>[4x]MSQHNEKNPHQHQSPLHDSSEAKPGMDSLAPEDGSHRPAAEPTPPGAQPTAPGSLKAPDTRNEKLNSLEDVRKGSENYALTTNQGVRIADDQNSLRAGSRGPTLLEDFILREKIAHFDHERIPERIVHARGSAAHGYFQPYKSLSDITKADFLSDPNKITPVFVRFSTVQGGAGSADTVRDIRGFATKFYTEEGIFDLVGNNTPIFFIQDAHKFPDFVHAVKPEPHWAIPQGQSAHDTFWDYVSLQP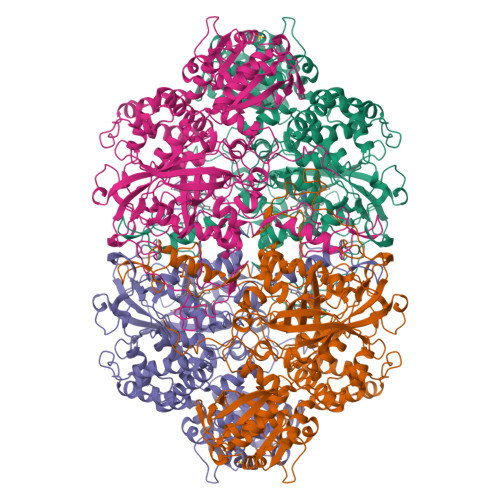ETLHNVMWAMSDRGIPRSYRTMEGFGIHTFRLINAEGKATFVRFHWKPLAGKASLVWDEAQKLTGRDPDFHRRELWEAIEAGDFPEYELGFQLIPEEDEFKFDFDLLDPTKLIPEELVPVQRVGKMVLNRNPDNFFAENEQAAFHPGHIVPGLDFTNDPLLQGRLYSYTDTQISRLGGPNFHEIPINRPTCPYHNFQRDGMHRMGIDTNPANYEPNSINDNWPRETPPGPKRGGFESYQERVEGNKVRERSPSFGEYYSHPRLFWLSQTPFEQRHIVDGFSFELSKVVRPYIRERVVDQLAHIDLTLAQAVAKNLGIELTDDQLNITPPPDVNGLKKDPSLSLYAIPDGDVKGRVVAILLNDEVRSADLLAILKALKAKGVHAKLLYSRMGEVTADDGTVLPIAATFAGAPSLTVDAVIVPCGNIADIADNGDANYYLMEAYKHLKPIALAGDARKFKATIKIADQGEEGIVEADSADGSFMDELLTLMAAHRVWSRIPKIDKIPA Mevalonate kinase is central to the isoprenoid biosynthesis pathway. Mevalonate kinases (MK) catalyse the phosphorylation of mevalonate. Mevalonate kinases belong to the GHMP kinase superfamily, which includes enzymes such as galactokinase, homoserine kinase, MK and phosphomevalonate kinase. The His tag was not resolved in the structure. Like all GHMP superfamily enzymes, each monomer is composed of two domains: an N-terminal domain and a C-terminal domain separated by a cleft.

In this work, we have identified, purified and characterized, both biochemically and structurally, two previously uncharacterized mevalonate kinases originating from the extremotolerant tardigrade R. varieornatus (Hashimoto et al., 2016; MKvar) and the psychrophilic archaeon M. burtonii (MKbur; Allen et al., 2009). As part of this study, the crystal structure of MKvar with mevalonate in the active site was determined to 2 Å resolution and the crystal structure of MKbur was determined to 2.2 Å resolution. A loop region between α3 and α4 in MKvar is not seen in the X-ray structure, suggesting high mobility of this loop; mobility in this region is also observed in some other MK structures. The N-terminal sections missing from eubacterial and archaeal MKs mostly form the two helices α2 and α3 in MKvar and can also be found in rat and human MK. A conserved Arg residue in MKrat (Arg241), corresponding to Arg261 in MKvar, was found to be essential in binding the tail of ATP and moves inside the active site upon binding the substrates; no equivalent arginine residue can be found in MKbur or MKmaz, where it is replaced by a serine. In MKvar, Thr119 and Ile215 align with Thr104 and Ile196, respectively, in human MK. The distance between Thr119 (the N-terminus of the α4 helix) and the ribose of the ATP molecule is ∼3 Å in MKvar, compared with a distance of ∼7 Å to the N-terminus of the α1 helix in MKbur. MKvar presents a classic feedback-inhibited profile, as well as inhibition by its own product, while MKbur, similar to many different archaeal MKs, does not appear to be significantly inhibited by FPP or GPP compounds.

>[2x]MHHHHHHGSMSNLRHLRVSAPGKIILHGEHAVVYQKTAVALSLGLRTRLDLTETTDGRISIIMDKFLQHTSWSVEELSKIIDKVKIDANNPETELDQELVEDLRMMTSGHHYQNGDGPAVGNPQAYSTQSVALVGFLYILVKLCKFSGKQRPPSIQISISSDIAISAGLGSSAAFAVCLSASLLSYLGIIVCDRKNCADVDGKLVPSADQLALINHWAFMVEKIVHGSASGVDNAVSTYGGSIKYRNNELTRIGSGLKLDVLIVDTHVQRDTKKMLDIVRHRRKLYPAITNPVLEAIDGISETSSKILQHGDGLPTGEEYEVIADLVRMNQNLLSTLGVSHPKLDVICETASRFGQAGKLTGAGGGGCAIVVLDPDMRQFEHLRESIIAEYRRMEFKPHLAELGGPGVLFHPVPGS>[4x]GSHMSVAQVATGSPRPGLFHLDSSVVDLSGDDFSRVHRVAPLCPWIVLFYNDGCGASRRYASTFSKFAGGLKVEHGKDALQIATAAAVNCASEVDLCRKYDINFVPRLFFFYPRDSCRSNEECGTSSLEHVAFENSHLEVDELESEVRRLVNKHMVVDDSLKERCIDMHFKLYTSKEELVKRSVSSTDESGRFVETTELYATDIAGAFFSAMHY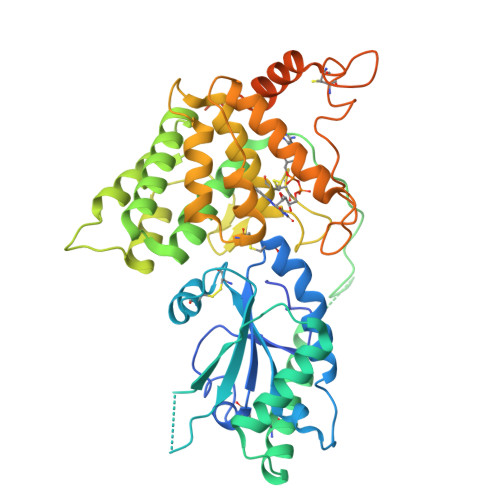DVSLVGTEPRERLTALEDFVLLVKDSLPSIGADGVVSALESITAERPFTVASWQDAVVKSGIPFDGSPRNVRWRTCRGSSPQYRGFPCGMWLLLHALTVNTPADRNVLEVIQNYIRYFFSCKESRDHFIQFNFSPNEDPVLQLWRAHNNVNARLANVKDGADPLVPKRQFPTLEACTECYDGAGNFIEAHVTGFLKQRYLWDPKAVGLMESNDDLNEVDPASKDANVGRNVESSGKGKGDGGARGNSKEVRSDHAG> MEQNGLDHDSRSSIDTTINDTQKTFLEFRSYTQLSEKLASSSSYTAPPLNEDGPKGVASAVSQGSESVVSWTTLTHVYSILGAYGGPTCLYPTATYFLMGTSKGCVLIFNYNEHLQTILVPTLSEDPSIHSIRSPVKSIVICSDGTHVAASYETGNICIWNLNVGYRVKPTSEPTNGMTPTPALPAVLHIDDHVNKEITGLDFFGARHTALIVSDRTGKVSLYNGYRRGFWQLVYNSKKILDVNSSKEKLIRSKLSPLISREKISTNLLSVLTTTHFALILLSP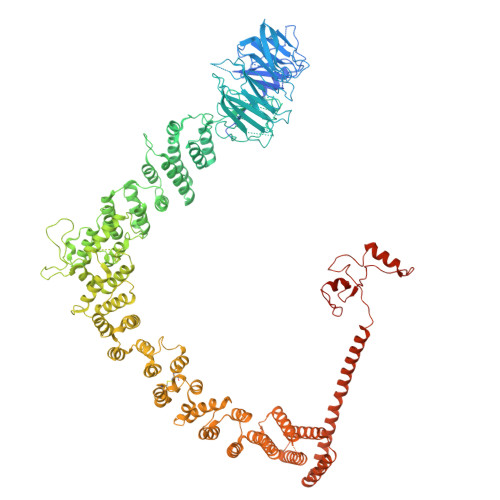HVSLMFQETVEPSVQNSLVVNSSISWTQNCSRVAYSVNNKISVISISSSDFNVQSASHSPEFAESILSIQWIDQLLLGVLTISHQFLVLHPQHDFKILLRLDFLIHDLMIPPNKYFVISRRSFYLLTNYSFKIGKFVSWSDITLRHILKGDYLGALEFIESLLQPYCPLANLLKLDNNTEERTKQLMEPFYNLSLAALRFLIKKDNADYNRVYQLLMVVVRVLQQSSKKLDSIPSLDVFLEQGLEFFELKDNAVYFEVVANIVAQGSVTSISPVLFRSIIDYYAKEENLKVIEDLIIMLNPTTLDVDLAVKLCQKYNLFDLLIYIWNKIFDDYQTPVVDLIYRISNQSEKCVIFNGPQVPPETTIFDYVTYILTGRQYPQNLSISPSDKCSKIQRELSAFIFSGFSIKWPSNSNHKLYICENPEEEPAFPYFHLLLKSNPSRFLAMLNEVFEASLFNDDNDMVASVGEAELVSRQYVIDLLLDAMKDTGNSDNIRVLVAIFIATSISKYPQFIKVSNQALDCVVNTICSSRVQGIYEISQIALESLLPYYHSRTTENFILELKEKNFNKVLFHIYKSENKYASALSLILETKDIEKEYNTDIVSITDYILKKCPPGSLECGKVTEVIETNFDLLLSRIGIEKCVTIFSDFDYNLHQEILEVKNEETQQKYLDKLFSTPNINNKVDKRLRNLHIELNCKYKSKREMILWLNGTVLSNAESLQILDLLNQDSNFEAAAIIHERLESFNLAVRDLLSFIEQCLNEGKTNISTLLESLRRAFDDCNSAGTEKKSCWILLITFLITLYGKYPSHDERKDLCNKLLQEAFLGLVRSKSSSQKDSGGEFWEIMSSVLEHQDVILMKVQDLKQLLLNVFNTYKLERSLSELIQKIIEDSSQDLVQQYRKFLSEGWSIHTDDCEICGKKIWGAGLDPLLFLAWENVQRHQDMISVDLKTPLVIFKCHHGFHQTCLENLAQKPDEYSCLICQTESNPKIVDYKDDDDKDYKDDDDKDYKDDDDK> MTTPISPPPQWS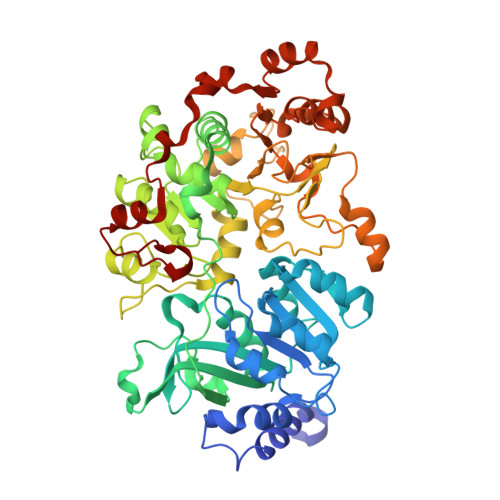RRRQEKQRRLERVRGLADGAVLPREGLVAALEALIAPGDRVVLEGNNQKQADFLSRSLARVDPGKLHDLHMIMPSVGRPEHLDLFELGIARKLDFSFSGPQSLRIGQLLEDGLLEIGAIHTYIELYARLVVDLIPNVALVAGFVADREGNVYTGPSTEDTPALVEPTAFSDGIVIVQVNRIVDDPRDLPRVDIPASWVDFVVEADQPFYIEPLFTRDPRHIKPVHVLMAMMAIRGIYQRHNVQSLNHGIGFNTAAIELILPTYGESLGLKGKICRHWTLNPHPTLIPAIESGWVESVHCFGTELGMEGYIAQRPDVFFTGRDGSLRSNRMFCQLAGQYAVDLFIGATLQVDGDGHSSTVTRGRLAGFGGAPNMGHDPRGRRHSTPAWLDMRGEPEALLERGRKLVVQMVETFQDGGKPTFVERLDALEVARQTGMPLAPVMIYGDDVTHVLTEEGIAYLYKARSLEERQAMIAAVAGISPIGLRHDPRETQRMRREGLIALPEDLGIRRTDASRELLAAKSIAELVEWSGGLYQPPARFRSW Here, we report phylogenetic analyses, combined with the selection and characterisation of five fungal AA7s, three of which belong to previously unexplored clades. We determined the crystal structures of FgChi7B and FgCelDH7C at resolutions of 2.4 and 1.6 Å, respectively. Both enzymes share the canonical AA7 fold comprising an FAD-binding F domain and a substrate-binding S domain that is formed by a central β-sheet flanked by α-helices. Moreover, the two enzymes share an aromatic cluster comprising: (i) the catalytic base tyrosine (FgCelDH7C Y454), (ii) a tyrosine/phenylalanine (FgCelDH7C F99) that stacks onto and stabilises the catalytic base, and (iii) an aromatic residue that stacks mainly onto the saccharide unit penultimate to the reducing end (FgCelDH7C F383).

The selected fungal sequences share 25–39% amino acid sequence identity and originate from Aspergillus nidulans (AnAA7A, clade I), Fusarium graminearum (FgCelDH7C, clade IIa and FgChi7B, clade Va), Magnaporthe oryzae (MoChi7A, clade Vb) and Polyporus brumalis (PbChi7A, clade VI). FgChi7B (clade Va), MoChi7A (clade Vb) and PbChi7A (clade VI) displayed the highest normalised rates (Vo/E) on chitooligosaccharides, followed by N-acetyl glucosamine (GlcNAc). The KM values of MoChi7A and PbChi7A towards GlcNAc were about 20-fold lower compared to FgChi7B, highlighting a marked difference in affinity for monosaccharides between these enzymes. All previously characterised AA7 oxidases are distinguished by a cysteinyl and histidyl bi-covalently tethered FAD cofactor. Thus, the isoalloxazine ring of the FAD cofactor in FgChi7B is bi-covalently anchored at the C6 atom to C162 Sγ (6-S-cysteinyl) and the 8α-methyl group to H102 Nδ1 (8α-N1-histidyl), akin to all previously determined AA7 structures.

> MFDFRLLLLCLGAFLTFTNASPSPYPQSSNAPAALNACLASKKVPYIPRDSAQWVKEVKPYNLRLAYTPAAIALPTTVKHISDAVKCGDQNKVRVSAKSGGHSYGSFGYGGENGHLVIVVDAMDTVTLNKDMSCTVQAGARLGHVATDLFQFGKRAIPHGSCPGVGIAGHALHGGYGFASRTHGLTLDTFLGATIVLTNGTIRYAADWEYYDLTWALRGAGSSFGIVAELGFQTFAAPETVTPFSIELDWNENEAVEGLLAMQKFAVTAPKELNMQIYMGPSGQTIQGVYYGTRANLNTALRPLLGDLGAQISTASTGGWIQMLNKYANGQALDQRRPYDQHSTFYSTSLMTKALTRNQVKSFARTLFDNMNDSDARHTWYILIDLFGGPNSAVTNAKTLFTDLPINSAFPHRDKLLLWQFSDHGNYATHANNGFTVLKRFRDSVTKTMADGDWGMYANYLDTQLSNEEAVKRYYGKSLPKLKKLKAELDPKDMFWNPQGIRPAAAHHHHHH~{N}-[(5~{S},8~{S},11~{S},15~{R})-8-[(4-fluorophenyl)methyl]-5-(hydroxymethyl)-2,7,10,14-tetrakis(oxidanylidene)-1,6,9,13-tetrazabicyclo[13.3.0]octadecan-11-yl]-5-methyl-1,2-oxazole-3-carboxamide | C27 H33 F N6 O7 | 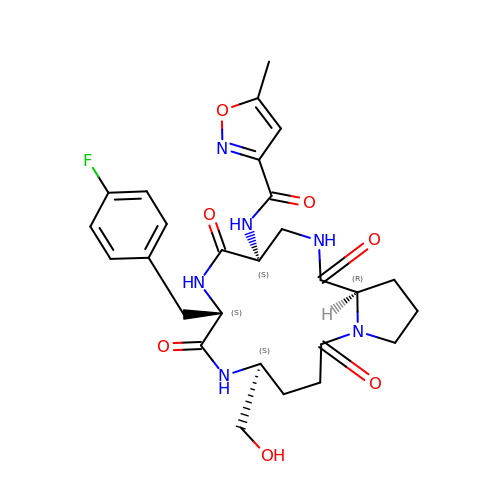XGIISLQJIYRWPH-BLKABHOGSA-N1,3,5-triazine-2,4,6-triol 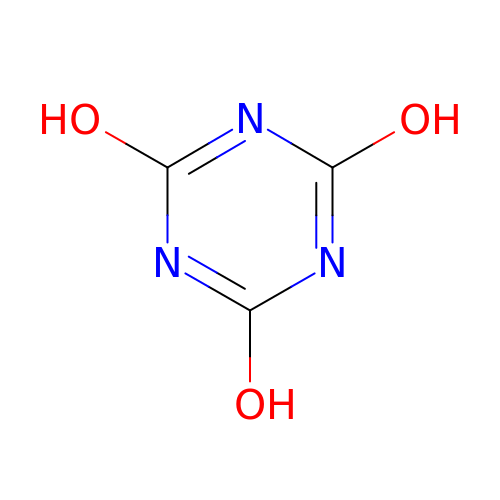| C3 H3 N3 O3 | ZFSLODLOARCGLH-UHFFFAOYSA-N Oligopeptidase B (OpB) is a two-domain, trypsin-like serine peptidase belonging to the S9 prolyloligopeptidase (POP) family. Two domains are linked by a hinge region that participates in the transition of the enzyme between two major states—closed and open—in which domains and residues of the catalytic triad are located close to each other and separated, respectively. In this study, we described for the first time the structures of bacterial OpB from S. proteomaculans (PSP) obtained by X-ray for an enzyme with a modified hinge region (PSPmod) and two of its derivatives. The enzymes were crystallized in the presence of spermine and adopted uncommon intermediate states in the crystal lattices.

Despite its small effect on thermal stability, the presence of Sp made it possible to obtain crystals suitable for X-ray analysis for PSPmod and its derivatives, PSPmodE125A and PSPmodS532A. The partial restoration of the catalytic activity of PSPmod was also achieved by the alanine substitution of Glu125 acidic residue from the β-propeller domain: PSPmodE125A possesses hydrolysis efficiency toward the substrates, from 19 to 26%, of PSP, demonstrating increases in hydrolysis efficiency (kcat/Km) over PSPmod by about 6- to 9-fold. According to our previous in silico modelling, Glu125 also participated in the putative interdomain SB network and its alanine substitution increased the activities of PSP toward BAPNA and dibasic substrates by about 8- and about 2-fold, respectively. PSPmod and two its derivatives (PSPmodE125A and PSPmodS532A) were crystallized in intermediate conformations, which are characterized by a disruption of the catalytic triad typical for ligand-free enzymes in open states, while domains’ closeness resembled closed states of ligand-bound POP. As a result, five, three and two bound Sp molecules were found in the structures of PSPmod, PSPmodE125A and PSPmodS532A, respectively. Sp701 is present in all structures, while Sp704—only in the PSPmod structure. The second and third Sp of PSPmodE125A occupy the positions of Sp702 and 705 in PSPmod, respectively. The PDDF profile of PSPmod has an intermediate width and reaches the minimum value for PSPmodE125A and PSP-Sp. This is consistent with the minimum distance between the center of mass of the domains and the maximum value of the buried surface area found in the crystal structure of PSPmodE125A compared to PSPmod. Analogously, if the differences in the SAXS profiles are determined by the ratio of the intermediate and open conformation in the solution, then the intermediate conformation dominates for PSPmodE125A.

> MTPPKAEKRPYPITTHGDTRVDDYYWLRDDERTDPQVLDYLQAENAFTDAALKPQQALRETLYEEMVARENLYFQSVPYVRHGYRYQTRFEPGNEYAIYVRQPQAESEHWDTLIDGNQRAEQRAFYTLGGLEVSPDNQKLAVAEDFLSRRQYDIRFKNLSDDSWTDEVLENTSGSFEWANDSATVYYVRKHAKTLLPYQVYRHVVGTDPQLDELIYEEQDDTFYVGLEKTTSDRFILIHLSSTTTSEILLLDADRADSTPQMFVPRRKDHEYGIDHYHQHFYIRSNKDGKNFGLYQSEQADEAQWQTLIAPRIEVMLEGFSLFRDWLVVEERSEGLTQLRQIHWQSGEVKRIAFDDPTYTTWLAYNPEPETELLRYGYSSMTTPTTLYELNLDSDERVMLKQQEVKNFTPENYRSERVWVKARDGVEVPVSLVYRHDSFARGTNPLMVYGYGSYGSSMDPAFSASRLSLLDRGFVFVLAHIRGGGELGQLWYEDGKLFKKQNTFNDFIDVTEALIAQGYGDAKRVFAMGGSAGGLLMGAVINQAPELFNGIVAQVPFVDVVTTMLDESIPLTTGEYDEWGNPNQQAYYDYILQYSPYDQVKAQDYPHMLVTTGLHDSQVQYWEPAKWVAKLRELKTDDRQLLLYTDMDSGHGGKSGRFKAYEDIALEYAFILALAE> ETFTVKMGADSGLLQFEPANVTVHP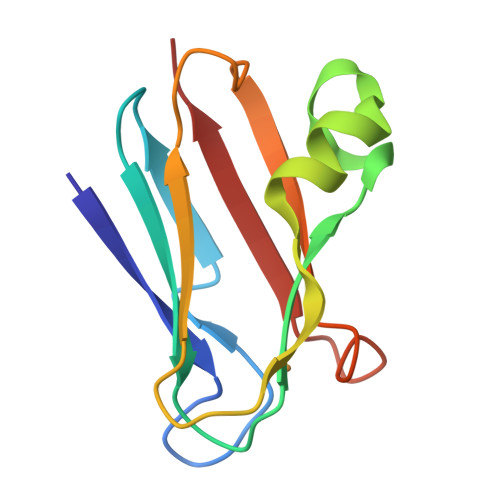GDTVKWVNNKLPPHNILFAAKQVPGASKELADKLSHSQLMFSPGESYEITFSSDFPAGTYTYYCAPHRGAGMVGKITVEG N-{[(3R)-pyrrolidin-3-yl]methyl}pyridin-2-amine 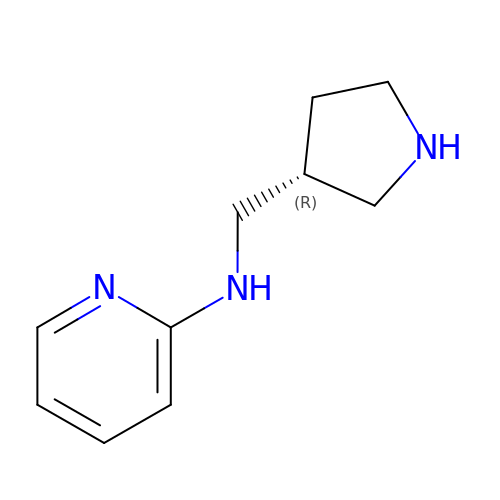| C10 H15 N3 | SHHXEJVQQWFIPM-SECBINFHSA-N> MLTMKDIIRDGHPTLRQKAAELELPLTKEEKETLIAMREFLVNSQDEEIAKRYGLRSGVGLAAPQINISKRMIAVLIPDDGSGKSYDYM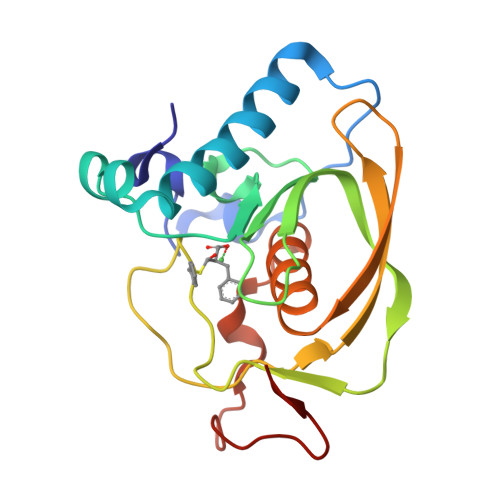LVNPKIVSHSVQEAYLPTGEGCLSVDDNVAGLVHRHNRITIKAKDIEGNDIQLRLKGYPAIVFQHEIDHLNGVMFYDHIDKNHPLQPHTDAVEVV> MAGQTTVDSRRQPPEEVDVLVVGAGFSGLYALYRLRELGRSVHVIETAGDVGGVWYWNRYPGARCDIESIEYCYSFSEEVLQEWNWTERYASQPEILRYINFVADKFDLRSGITFHTTVTAAAFDEATNTWTVDTNHGDRIRARYLIMASGQLSVPQLPNFPGLKDFAGNLYHTGNWPHEPVDFSGQRVGVIGTGSSGIQVSPQIAKQAAELFVFQRTPHFAVPARNAPLDPEFLADLKKRYAEFREESRNTPGGTH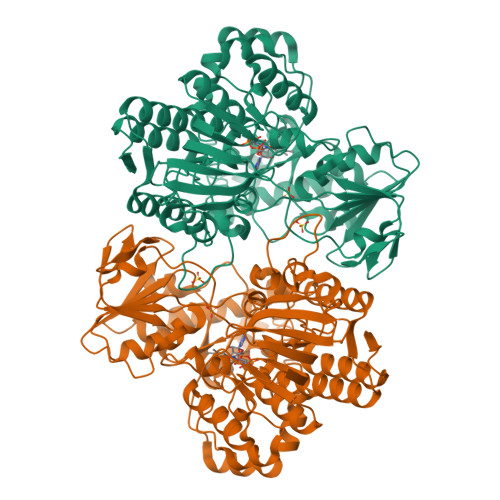RYQGPKSALEVSDEELVETLERYWQEGGPDILAAYRDILRDRDANERVAEFIRNKIRNTVRDPEVAERLVPKGYPFGTKRLILEIDYYEMFNRDNVHLVDTLSAPIETITPRGVRTSEREYELDSLVLATGFDALTGALFKIDIRGVGNVALKEKWAAGPRTYLGLSTAGFPNLFFIAGPGSPSALSNGLVSIEQHVEWVTDHIAYMFKNGLTRSEAVLEKEDEWVEHVNEIADETLYPMTASWYTGANVPGKPRVFMLYVGGFHRYRQICDEVAAKGYEGFVLT A class I chitinase from the carnivorous sundew plant Drosera adelae was successfully expressed in the methylotrophic yeast Pichia pastoris and efficiently purified using a chitin affinity column. Enzymatic activity assays revealed that the enzyme showed a specific activity of 235.3 ± 10.2 U·mg−1. In D. adelae chitinase, a characteristic tyrosine cluster consisting of Tyr174, Tyr199, and Tyr201 formed a unique structural feature that enabled recognition of the (GlcNAc)4 substrate. The hevein domain structures further indicated that the tyrosine cluster (Tyr41, Tyr43, Tyr50) in D. adelae chitinase may be involved in hydrogen bonding and CH/π interactions with (GlcNAc)3.

Crystallization of wild‐type and E167Q catalytic mutant chitinases yielded needle‐like microcrystals. X‐ray diffraction experiments were performed, and high‐resolution datasets were obtained at 1.73 Å and 1.57 Å, respectively. Structural analysis of diffraction data revealed that only the catalytic domain could be resolved in both crystal forms. Using AutoDock Vina, we performed docking simulations of two (GlcNAc)4 molecules at eight subsites (+4 to −4) of the catalytic domain of D. adelae chitinase to investigate their binding energies and conformations. Further, the structure of the chitin‐binding domain (hevein domain), which could not be resolved by X‐ray crystallography, was predicted using alphafold.

>[2x]DVSSIITSQIFNQMLLHRNDNACPANGFYSYQAFINAARKFSGFGTTGDTNTRKNELAAFFGQTSHETTGGWSTAPDGPYAWGYCFKQEQGNPGDYCVPSSTYPCAPGKKYYGRGPIQISYNYNYGLCGAAINQPLLSNPGLVASDADISFETAIWFWMTPQGNKPSCHAVATGQWNPSSADQAAGRVPGYGVITNIINGGVECGQGEKAEVANRIGFYQRYCSIFGISPGQNLDCYNQRPFS pyridin-4-ol | C5 H5 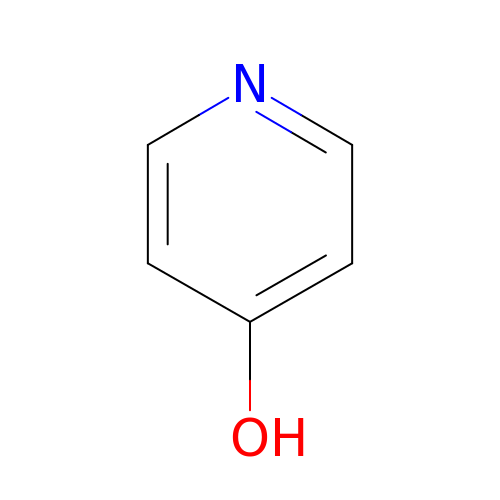N O | GCNTZFIIOFTKIY-UHFFFAOYSA-N>GPLGSMSVAGLKKQFHKATQKVSEKVGGAEGTKLDDDFKEMERKVDVTSRAVMEIMTKTIEYLQPNPASRAKLSMINTMSKIRGQEKGPGYPQAEALLAEAMLKFGRELGDDCNFGP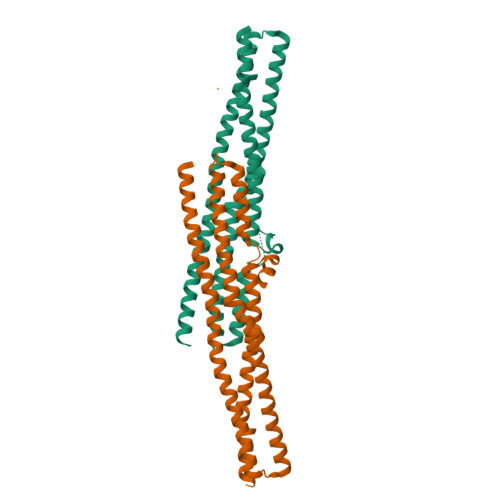ALGEVGEAMRELSEVKDSLDIEVKQNFIDPLQNLHDKDLREIQSALQHHLKKLEGRRLDFDYKKKRQGKIPDEELRQALEKFDESKEIAESSMFNLLEMDIEQVSQLSALVQAQLEYHKQAVQILQQVTVRLEERIRQA[4x]> ANKTRELCMKSLEHAKVD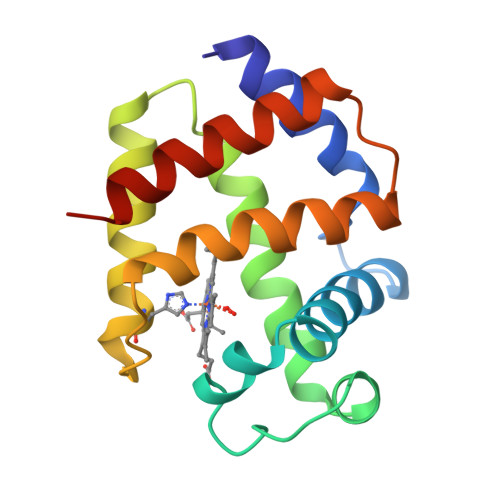TSNEARQDGIDLYKHMFENYPPLRKYFKSREEYTAEDVQNDPFFAKQGQKILLACHVLCATYDDRETFNAYTRELLDRHARDHVHMPPEVWTDFWKLFEEYLGKKTTLDEPTKQAWHEIGREFAKEINKHGR> MGNTTSDRVSGERHGAKAARSEGAGGHAPGKEHKIMVGSTDDPSVFSLPDSKLPGDKEFVSWQQDLEDSVKPTQQARPTVIRWSEGGKEVFISGSFNNWSTKIPLIKSHNDFVAILDLPEGEHQYKFFVDGQWVHDPSEPVVTSQLGTINNLIHVKKSDFEVFDALKLDSMESSETSCRDLSSSPPGPYGQEMYAFRSEERFKSPPILPPHLLQVILNKDTNISCDPALLPEPNHVMLNHLYALSIKDSVMVLSATHRYK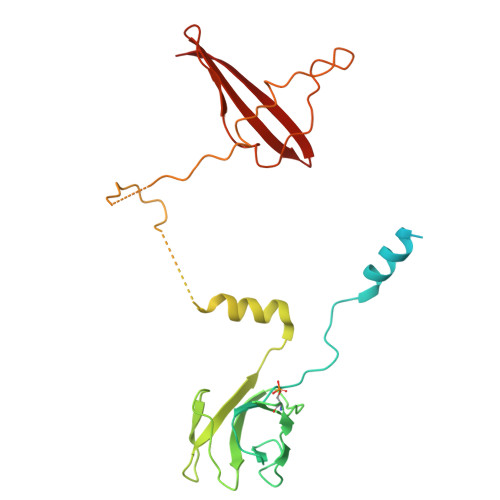KKYVTTLLYKPI Enmetazobactam derived trans-enamine 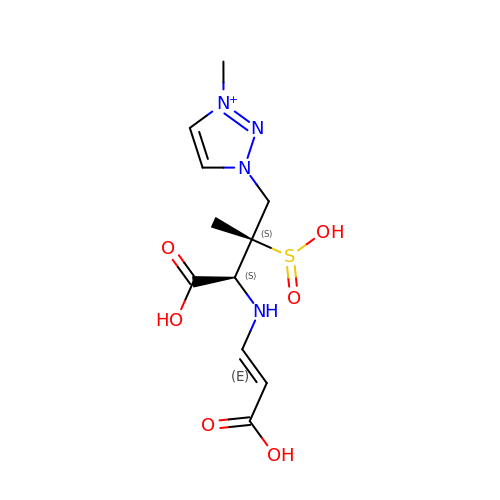adduct | C11 H17 N4 O6 S | VVXNTAXAJHAELU-UEVFTQGLSA-O>QGMTVGTYAELASVFAALSDETRWEILTELGRADQSASSL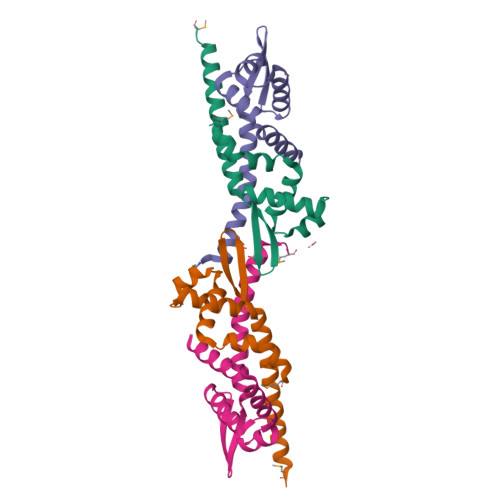ATRLPVSRQAIAKHLNALQACGLVESVKVGREIRYRALGAELNKTARTLERIGAEWDRRLAAIKQIAESMEEGS[4x]>[2x]VLAQNKADVISKCLDDAGIRNVIDTDSSWAQETVMFQKRLKPDPEAIAFPENSDEVASALKCARESKVKANALGPAHSFQGNGFGIPGNLVINMAAFDEVSYDKKSTLLTFGGGTHVGPVQKYLWDTAGRHVPHVRGAHVGVTGSSIGGGFGTTSRYLGTPMDNLVEIQYMLYNGTIVNAKKGSDLFWAAQGAGASFGIILSTKTKTFKPQFDKAINFTLSMGDLTPEAGAKALVAIQDYSLSKDCPDTWAFRWNIMAPPYDGTGYFYGNPSSFDSVMAPLVKKLKTISSNTAVKSTVLPWWDLEVAVAGPGMNQPNGGALGGRSFYTQSLTTTTDHPLTVKQAQILFEGTTLAFNRTDMTKFGYMDLWGGVSRSIKDSDTAYAHGKNLWLIRWDANAIGAYPSDGISYMRASIKPFEDSLVKGGAKLRGFVNYADTELTEKEWSSRLYDGNFERLKQIKARYDPEGLFINHRQSIPLPAAAHHHHHH

Here, we report phylogenetic analyses, combined with the selection and characterisation of five fungal AA7s, three of which belong to previously unexplored clades. We determined the crystal structures of FgChi7B and FgCelDH7C at resolutions of 2.4 and 1.6 Å, respectively. Both enzymes share the canonical AA7 fold comprising an FAD-binding F domain and a substrate-binding S domain that is formed by a central β-sheet flanked by α-helices. Moreover, the two enzymes share an aromatic cluster comprising: (i) the catalytic base tyrosine (FgCelDH7C Y454), (ii) a tyrosine/phenylalanine (FgCelDH7C F99) that stacks onto and stabilises the catalytic base, and (iii) an aromatic residue that stacks mainly onto the saccharide unit penultimate to the reducing end (FgCelDH7C F383).

By contrast, FgCelDH7C acted as a dehydrogenase with a preference for cellooligosaccharides with kcat values of 32–42 s−1 and the highest catalytic efficiency on cellotriose. By contrast, the structure of FgCelDH7C revealed a unique active site architecture, as compared to all hitherto available AA7 structures. The first notable overall structural difference is that a loop (residues Q335-F346) that flanks the active site in FgCelDH7C appears shorter due to a preceding helical segment that folds away from the active site, which provides a less occluded and more solvent-exposed FAD-cofactor compared to FgChi7B and all hitherto reported AA7 structures. Strikingly, the mode of FAD-anchoring represents a second unique characteristic distinguishing FgCelDH7C from the other AA7 structures. Thus, the isoalloxazine ring of the FAD cofactor in FgChi7B is bi-covalently anchored at the C6 atom to C162 Sγ (6-S-cysteinyl) and the 8α-methyl group to H102 Nδ1 (8α-N1-histidyl), akin to all previously determined AA7 structures. By contrast, FgCelDH7C is mono-covalently histidyl-tethered due to the substitution of the FAD-tethering cysteine to a glycine. A third structural signature of FgCelDH7C, compared to all available AA7 structures, is the substitution of a histidine residue facing the isoalloxazine ring in the FAD-binding domain to a serine (S165). A fourth different motif in FgCelDH7C entails four arginine residues that protrude into the substrate-binding pocket, providing a distinctively positive charged milieu compared to other structurally characterised AA7s. On the other hand, the uniquely open and positively charged active site of FgCelDH7C, compared to structural homologues, may favour the accommodation of organic electron acceptors to promote the dehydrogenase oxidative half reaction. We have shown that FgCelDH7C potentiates LPMO-catalysed cellulose degradation in the absence of any exogenous reductant.> QD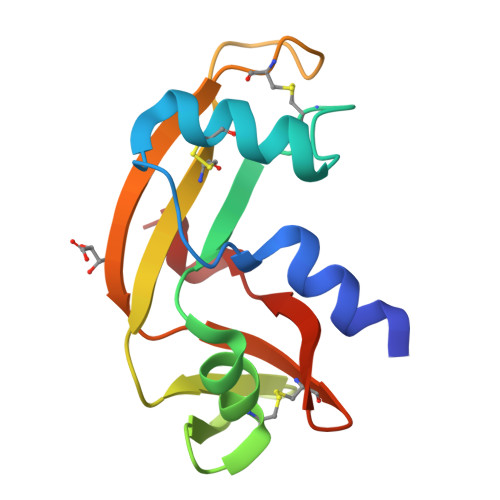NSRYTHFLTQHYDAIPQGRDDRYCESIMRRRGLTSPCKDINTFIHGNKRSIKAICENKNGNPHRENLRISKSSFQVTTCKLHGGSPWPPCQYRATAGFRNVVVACENGLPVHLDQSIFRRP> GSSGSSGMIKEYRTIKEVVGPLMAVEKVSGVKYEELIEVRMQNGEIRRGQVLEVQEDKAMVQIFEGTSGINLKNSSVRFLGHPLQLGVSEDMIGRVFDGLGRPKDNGPEILPEKYLDINGEVINPIARDYPDEFIQTGISAIDHLNTLVRGQKLPVFSGSGLPHKELAAQIARQATVLDSSDDFAVVFAAIGITFEEAEFFMEDFRQTGAIDRSVMFMNLANDPAIERIATPRMALTAAEYLAYEKGMHVLVIMTDMTNYAEALREISAARREVPGRRGYPGYLYTNLATLFERAGRIRGLKGSVTQIPILTMPEDDKTHPIPDLTGYITE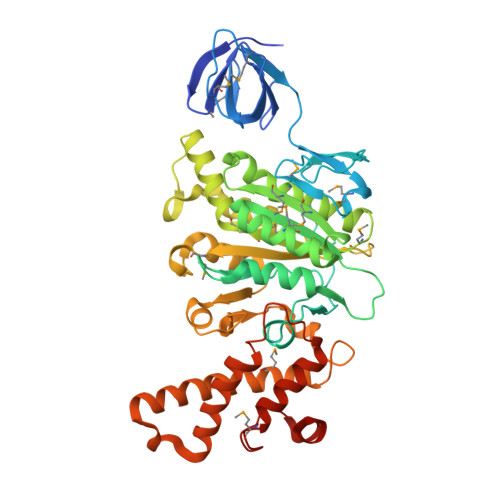GQIILTRELYKSGIQPPIDVLPSLSRLKDKGTGAGKTREDHAATMNQLFAAYAQGKQAKELAVVLGESALSDIDKIYAKFAERFENEYVNQGFYTNRTITETLDLGWELLAMLPRTELKRIKDDLLDKYLPEGK> MSSSIREEVHRHLGTVALMQPALHQQTHAPAPTEITHTLFRAYTRVPHDVGGEADVPIEYHEKEEEIWELNTFATCECLAWRGVWTAEERRRKQNCDVGQTVYLGMPYYGRWLLTAARILVDKQFVTLTELHNKIVEMRERVASGQG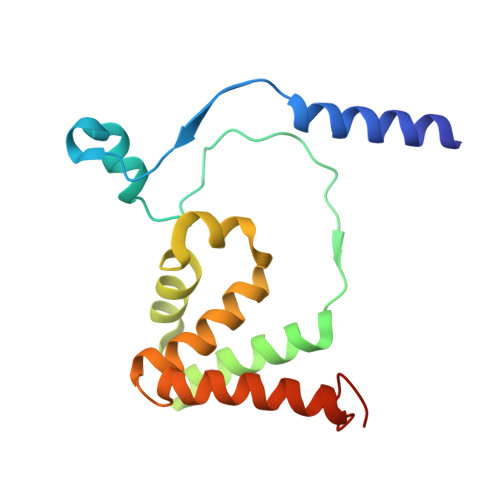LGEYLPPKAK> MGSADASTFLNRVCGVSAARLTPCGTGTSTDVVYRAFDIYNEKVAGFAKFLKTNCCRFQEKDEEGNLLDSYFVVKRHTMSNYQHEETIYNLVKDCPAVAVHDFFKFRVDGDMVPHISRQRLTKYTMADLVYALRHFDEGNCDTLKEILVTYNCCDDDYFNKKDWYDFVENPDILRVYANLGERVRQSLLKTVQFCDAMRDAGIVGVLTLDNQDLNGNWYDFGDFVQVAPGCGVPIVDSYYSLLMPILTLTRALAAESHMDADLAKPLIKWDLLKYDFTEERLCLFDRYFKYWDQTYHPNCINCLDDRCILHCANFNVLFSTVFPPTSFGPLVRKIFVDGVPFVVSTGYHFRELGVVHNQDVNLHSSRLSFKELLVYAADPAM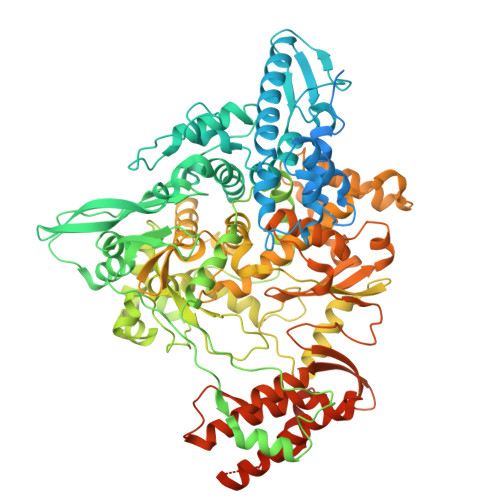HAASGNLLLDKRTTCFSVAALTNNVAFQTVKPGNFNKDFYDFAVSKGFFKEGSSVELKHFFFAQDGNAAISDYDYYRYNLPTMCDIRQLLFVVEVVDKYFDCYDGGCINANQVIVNNLDKSAGFPFNKWGKARLYYDSMSYEDQDALFAYTKRNVIPTITQMNLKYAISAKNRARTVAGVSICSTMTNRQFHQKLLKSIAATRGATVVIGTSKFYGGWHNMLKTVYSDVETPHLMGWDYPKCDRAMPNMLRIMASLVLARKHNTCCNLSHRFYRLANECAQVLSEMVMCGGSLYVKPGGTSSGDATTAYANSVFNICQAVTANVNALLSTDGNKIADKYVRNLQHRLYECLYRNRDVDHEFVDEFYAYLRKHFSMMILSDDAVVCYNSNYAAQGLVASIKNFKAVLYYQNNVFMSEAKCWTETDLTKGPHEFCSQHTMLVKQGDDYVYLPYPDPSRILGAGCFVDDIVKTDGTLMIERFVSLAIDAYPLTKHPNQEYADVFHLYLQYIRKLHDELTGHMLDMYSVMLTNDNTSRYWEPEFYEAMYTPHTVLLVPRGSGHHHHHHAWSHPQFEK> GPGSAPGPSRIADYLLLPLAER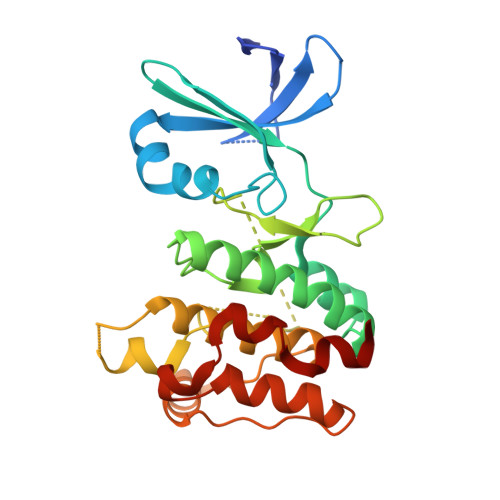EHVSRALCIHTGRELRCKVFPIKHYQDKIRPYIQLPSHSNITGIVEVILGETKAYVFFEKDFGDMHSYVRSRKRLREEEAARLFKQIVSAVAHCHQSAIVLGDLKLRKFVFSTEERTQLRLESLEDTHIMKGEDDALSDKHGCPAYVSPEILNTTGTYSGKAADVWSLGVMLYTLLVGRYPFHDSDPSALFSKIRRGQFCIPEHISPKARCLIRSLLRREPSERLTAPEILLHPWFESVLE> MKRKVLLIPLIIFLAIAAALLWQLARNAEGDDPTNLESALIGKPVPKFRLESLDNPGQFYQADVLTQGKPVLLNVWATWCPTCRAEHQYLNQLSAQGIRVVGMNYKDDRQKAISWLKELGNPYALSLFDGDGMLGLDLGVYGAPETFLIDGNGIIRY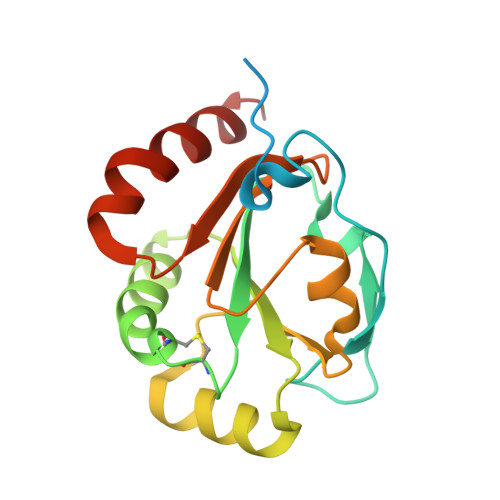RHAGDLNPRVWEEEIKPLWEKYSKEAAQ>[2x]GAMDPREVILCKDQDGKIGLRLKSIDNGIFVQLVQANSPASLVGLRFGDQVLQINGENCAGWSSDKAHKVLKQAFGEKITMTIRDRPFERTITM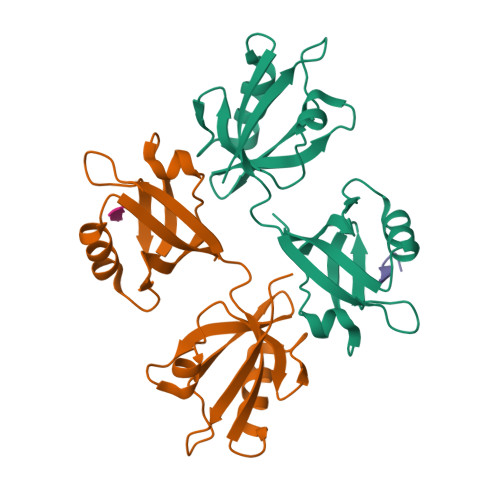HKDSTGHVGFIFKNGKITSIVKDSSAARNGLLTEHNICEINGQNVIGLKDSQIADILSTSGTVVTITIMPAF;>[2x]LGKKPIYKKAPTNEFYA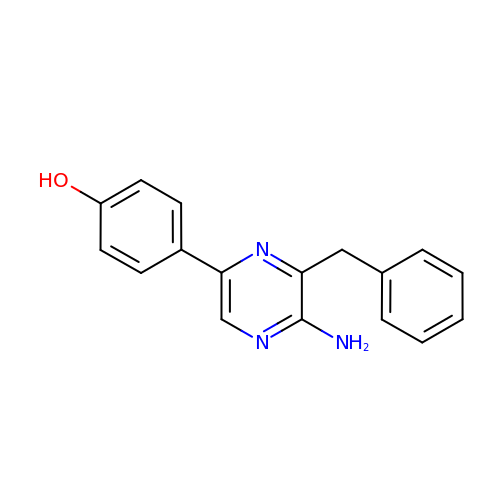4-[5-azanyl-6-(phenylmethyl)pyrazin-2-yl]phenol | C17 H15 N3 O | BWNPYAKFDUFNND-UHFFFAOYSA-N> MAHRSRCNCNDTSNSNGSQHGINLPLRKIDTYDPCVNCRVKPHLCPKPHPCPKPENLEADIVIIGAGAAGCVLAYYLTKFSDLKIILLEAGHTHFNDPVVTDPMGFFGKYNPPNENIRMSQNPSYAWQPALEPDTGAYSMRNVVAHGLAVGGSTAINQLNYIVGGRTVFDNDWPTGWKYDDIKKYFRRVLADISPIRDGTKVNLTNTILESMRVLA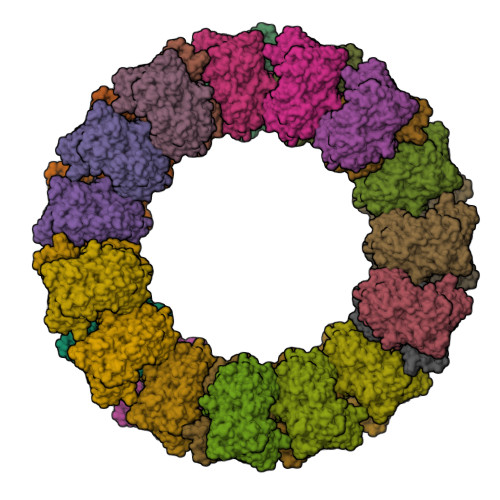DQQVSSGVPVDFLINKATGGLPNIEQTYQGAPIVNLNDYEGINSVCGFKSYYVGVNQLSDGSYIRKYAGNTYLNSYYVDSNGFGIGKFSNLRVISDAVVDRIHFEGQRAVSVTYIDKKGNLHSVKVHKEVEICSGSFFTPTILQRSGIGDFSYLSSIGVPDLVYNNPLVGQGLRNHYSPITQVSVTGPDAAAFLSNTAAGPTNMSFRGAGMLGYHKLEPNKPSNAGSVTYRKYELLVTGGVAISADQQYLSGISSSTGNYFALIADDIRFAPVGYIKIGTPNFPRDTPKIFFNTFVNYTPTTDPADQQWPVAQKTLAPLISALLGYDAIYQIVQQMKVVAVNAGFNVTLQMAYPPNDLLVELHNGLNTYGINWWHYFVPSLVNDDTPAGKLFASTLSKLSYYPRSGAHLDSHQSCSCSIGGTVDTELKVIGVENVRVTDLSAAPHPPGGNTWCTAAMIGARATDLILGKPLVANLPPEDVPVFTTS>TDTFQMFWLDYCEVNNTLILFGKVKLKDDNCVSAMVQINGLCRELFFLPREGKTPTDIHEEIIPLLMDKYGLDNIRAKPQKMKYSFELPDIPSESDYLKVLLPYQTPKSSRDTIPSDLSSDTFYHVFGGNSNIFESFVIQNRIMGPCWLDIKGADFNSIRNASHCAVEVSVDKPQNITPTTTKTMPNLRCLSLSIQTLMNPKENKQEIVSITLSAYRNISLDSPIPENIKPDDLCTLVRPPQSTSFPLGLAALAKQKLPGRVRLFNNEKAMLSCFCAMLKVEDPDVIIGHRLQNVYLDVLAHRMHDLNIPTFSSIGRRLRRTWPEKFGRGNSNMNHFFISDICSGRLICDIANEMGQSLTPKCQSWDLSEMYQVTCEKEHKPLDIDYQNPQYQNDVNSMTMALQENITNCMISAEVSYRIQLLTLTKQLTNLAGNAWAQTLGGTRAGRNEYILLHEFSRNGFIVPDKEGNRSRAQKQRQNEENADAPVNSKKAKYQGGLVFEPEKGLHKNYVLVMDFNSLYPSIIQEFNICFTTVDRNKEDIDELPSVPPSEVDQGVLPRLLANLVDRRREVKKVMKTETDPHKRVQCDIRQQALKLTANSMYGCLGYVNSRFYAKPLAMLVTNKGREILMNTRQLAESMNLLVVYGDTDSVMIDTGCDNYADAIKIGLGFKRLVNERYRLLEIDIDNVFKKLLLHAKKKYAALTVNLDKNGNGTTVLEVKGLDMKRREFCPLSRDVSIHVLNTILSDKDPEEALQEVYDYLEDIRIKVETNNIRIDKYKINMKLSKDPKAYPGGKNMPAVQVALRMRKAGRVVKAGSVITFVITKQDEIDNAADTPALSVAERAHALNEVMIKSNNLIPDPQYYLEKQIFAPVERLLERIDSFNVVRLSEALGLDSKKYFRREGGNNNG[2x]

The eukaryotic primase is a heterodimer of catalytic and regulatory subunits that is associated with the catalytic subunit of Pol α and its accessory B subunit in a constitutive heterotetrameric assembly, the Pol α/primase complex. In contrast, the Pol α/primase complex produces longer, composite RNA-DNA primers that result from the concerted enzymatic activities of primase and Pol α (Chang et al., 1984; Hu et al., 1984; Singh, et al., 1986). We have determined crystal structures of the catalytic core (349–1258; 910 amino acids) of yeast Pol α in unliganded form (apo), bound to an RNA primer/DNA template duplex (binary complex) and in a productive complex with RNA primer/DNA template and incoming dGTP (ternary complex). The catalytic region of Pol α adopts the universal ‘right-hand' DNA polymerase fold consisting of a palm domain harboring the active site, a fingers domain that interacts with the incoming nucleotide and a thumb domain that grips the primer-template duplex.

Rotation of the palm domain is accompanied by a conformational rearrangement of region II that is necessary in order to accommodate the phosphoribose moiety of the incoming nucleotide. The two copies of binary complex present in the asymmetric unit of the crystals capture intermediate states of the transition, as in one binary complex the conformation of region II is apo-like, whereas in the second copy region II adopts a conformation akin to that observed in the ternary complex. The range of positions adopted by the palm domain in the apo, binary and ternary complex structures suggests that adoption of an active conformation by Pol α might require a wider set of conformational rearrangements than predicted by current models of DNA polymerase activity. The observed movement of the palm domain could participate in a ‘ratchet' mechanism for unidirectional translocation of Pol α, as return of the palm domain to the apo conformation after catalysis would propel the polymerase forward onto the next templating base. Interestingly, site-specific mutations of Ser863 in region II of human Pol α (Ser867 of yeast Pol α), which acts as the pivot during rotation of the palm domain, cause a drastic reduction in the specific activity of the polymerase without changing its kinetic parameters, in agreement with a potential structural role of this serine residue in DNA polymerisation.> SSTSLLFEQLNFLILVAAEAELPIAHSTRKLLMDNSCNNCQIYELYNENLKDVKTDKDWFMNKFGPQTVHFVISNTINFPFYKIVYFDLLIPVVSHTWVQDSVKTKRHLRTNMYSPNPFHLLRDCQVYISKSSFNKCEYILYSDLLHLLGGTLVNYISNRTTHVIVQSPQDPIIATVSKLTFGSFSSSSTNKHTEKPLREWKFVYPIWILYHFKMAKPLKGELATLCELDMQDTSEEQLFAKWEEVIGDKQTSSSQLTLHPNKT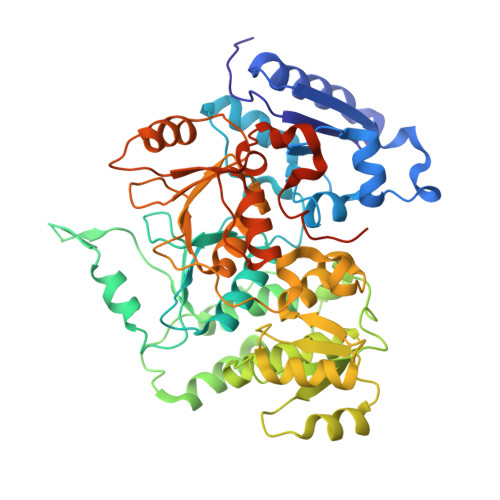LFKNHHFAISPDLNFFTPLYWFLKGFIEDLDGKVTPLSFSDDLKSVYQAFPDIDCYIGHSANSPILEKTKSIKPEIHVGNVSWLFYMFALQKFTPVSQCKLIHQPFHAKLFTSKELTVAYTNYFGSQRFYIQRLVEILGGLSTPELTRKNTHLITKSTIGKKFKVAKKWSLDPQNAIIVTNHMWLEQCYMNNSKLNPKDSRFQNFKLDDNMGWNIGQIGMDHSSLPTPKNLSMVTYDTQSISEKPPPTN>[4x]MKV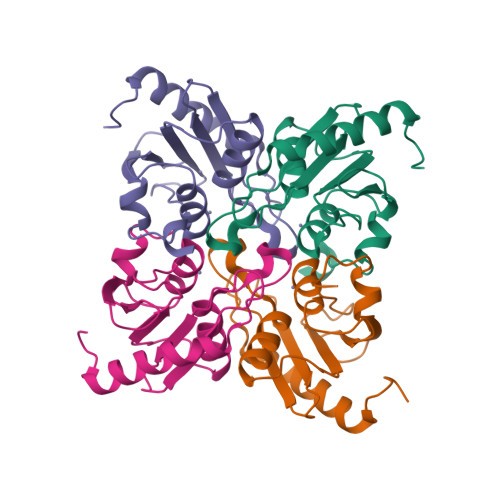GGIEDRQLEALKRAALKACELSYSPYSHFRVGCSILTNNDVIFTGANVENASYSNCICAERSAMIQVLMAGHRSGWKCMVICGDSEDQCVSPCGVCRQFINEFVVKDFPIVMLNSTGSRSKVMTMGELLPMAFGPSHLN> VVGGTEAQRNSWPSQISLQYRSGSSWAHTCGGTLIRQNWVMTAAHCVDRELTFRVVVGEHNLNQNNGTEQYVGVQKIVVHPYWNTDDVAAGYDIALLRL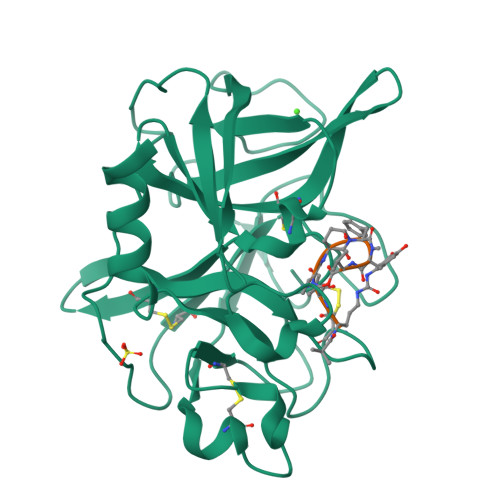AQSVTLNSYVQLGVLPRAGTILANNSPCYITGWGLTRTNGQLAQTLQQAYLPTVDYAICSSSSYWGSTVKNSMVCAGGDGVRSGCQGDSGGPLHCLVNGQYAVHGVTSFVSRLGCNVTRKPTVFTRVSAYISWINNVIASN;> XRTTEFYV2,5-dichloro-1H-benzimidazole | C7 H4 Cl2 N2 | 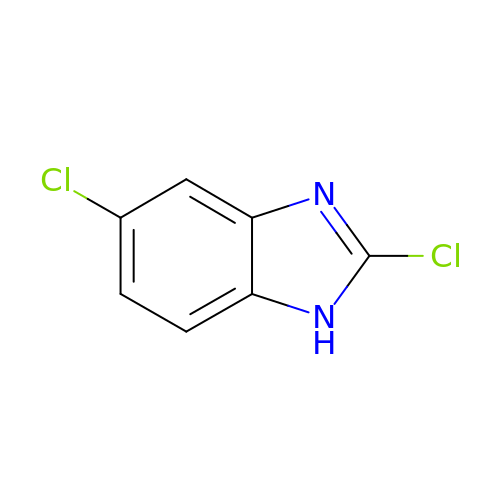LLIARSREYVCQHL-UHFFFAOYSA-N An oxidative system was recently discovered in which extracellular flavocytochromes, that is, cellobiose dehydrogenases (CDHs), cooperate with copper-dependent lytic polysaccharide monooxygenases (LPMOs)8910111213 to catalyse redox-mediated glycosidic bond cleavage in crystalline cellulose, hemicelluloses and starch. CDHs are large flavocytochromes containing a haem b-binding cytochrome domain (CYT) connected by a long, flexible linker to a flavin adenine dinucleotide (FAD)-binding dehydrogenase domain (DH). The DH domain oxidizes cellobiose at the C1 position to cellobiono-1,5-lactone with reduction of FAD. The ensuing step involves inter-domain electron transfer (IET) from the reduced FAD to CYT haem b, presumably by single electron-transfer (ET) events, followed by ET from CYT to external electron acceptors such as LPMOs.

We observed that crystals of native, full-length NcCDH typically lacked interpretable density for the CYT domains. Data from one platinum-soaked crystal offered better-defined electron density for the CYT domains, which allowed us to model both NcCDH molecules in the asymmetric unit. The overall weak density for the CYT domains suggests significant flexibility in the linker regions. The two non-crystallographically (NCS)-related molecules are present as two ‘open' states with different conformations of the flexible linkers and different relative orientations of the CYT and DH domains. The haem b is fully exposed and accessible in both open-state models. The crystal and solution structures of two closely related class-II CDHs revealed pronounced flexibility of the linker between the CYT and DH domains to allow the efficient association of the haem b with both the FAD electron donor (closed state) and external protein electron acceptors such as LPMO (open states). Overall, NcCDH has fewer negative surface residues but displays a similar trend of negative charges clustering near the channel entrance.

>QTAPKTFTHPDTGIVFNTWSASDSQTKGGFTVGMALPSNALTTDATEFIGYLECSSAKNGANSGWCGVSLRGAMTNNLLITAWPSDGEVYTNLMFATGYAMPKNYAGDAKITQIASSVNATHFTLVFRCQNCLSWDQDGVTGGISTSNKGAQLGWVQAFPSPGNPTCPTQITLSQHDNGMGQWGAAFDSNIANPSYTAWAAKATKTVTGTCSGPVTTSIAATPVPTGVSFDYIVVGGGAGGIPVADKLSESGKSVLLIEKGFASTGEHGGTLKPEWLNNTSLTRFDVPGLCNQIWKDSDGIACSDTDQMAGCVLGGGTAINAGLWYKPYTKDWDYLFPSGWKGSDIAGATSRALSRIPGTTTPSQDGKRYLQQGFEVLANGLKASGWKEVDSLKDSEQKNRTFSHTSYMYINGERGGPLATYLVSAKKRSNFKLWLNTAVKRVIREGGHITGVEVEAFRNGGYSGIIPVTNTTGRVVLSAGTFGSAKILLRSGIGPKDQLEVVKASADGPTMVSNSSWIDLPVGHNLVDHTNTDTVIQHNNVTFYDFYKAWDNPNTTDMNLYLNGRSGIFAQAAPNIGPLFWEEITGADGIVRQLHWTARVEGSFETPDGYAMTMSQYLGRGATSRGRMTLSPTLNTVVSDLPYLKDPNDKAAVVQGIVNLQKALANVKGLTWAYPSANQTAADFVDKQPVTYQSRRSNHWMGTNKMGTDDGRSGGTAVVDTNTRVYGTDNLYVVDASIFPGVPTTNPTAYIVVAAEHAAAKILAQPANEAVPKWGWCGGPTYTGSQTCQAPYKCEKQNDWYWQCV[2x]The traffic ATPase PilF from Thermus thermophilus is important for type IV pilus biogenesis, twitching motility, surface attachment, and natural DNA-uptake and contains three consecutive homologous GPSII domains. The N-terminal part of PilF harbors a remarkable arrangement of three successive general secretory pathway II (GSPII) domains (GSPII-A to GSPII-C) with high sequence similarity to each other. Interestingly, we find that PilF binds only two molecules of c-di-GMP with different affinities and that the c-di-GMP–binding activities can be attributed to the GSPII-B and GSPII-C domains. Remarkably, the GSPII-B domain binds c-di-GMP with a KD of only 6 nM and thus with an affinity ∼ 83fold higher than MshEN.

To further test if in general a hydrophobic interaction is indeed beneficial to high affinity c-di-GMP binding or if this effect is lysine specific, we created the K167L PilF159-302 variant and characterized its c-di-GMP–binding affinity. Remarkably, the ITC measurement with PilF159-302 K167L yielded an even lower KD value of 2 ± 0.3 nM than WT-PilF159-302 showing that the large hydrophobic side chain L167 might improve c-di-GMP binding of PilF159-302 even further. Thus, we crystallized the PilF159-302 K167L variant, which yielded crystals diffracting to 1.9 Å with the protein chain being traceable from residue 161 to 301 with no Ramachandran plot outliers. The L167 leucine side chain is well resolved and in a similar conformation in both chains of the asymmetric unit and involved in an extensive hydrophobic stacking interaction with the c-di-GMP guanine base. Moreover, a large hydrophobic residue at the very first position of the c-di-GMP–binding motif is apparently thermodynamically and dynamically beneficial for very high affinity c-di-GMP binding.

>[2x]GSSGEGQKDLLLGELLLQKGWISREALEEALVEQEKTGDLLGRILVRKGLPEEALYRALAEQKGLEFLESTEGIVPDPSAALLLLRSDALRYGAVPIGFQNGEVEVVLSDPRHKEAVAQLLNRPARFYLALPQAWEELFRRAYPQK> MLLHEFGLLESPKALEEAPWPPPEGAFVGFVLSRKEPMWADLLALAAARGGRVHRAPEPYKALRDLKEARGLLAKDLSVLALREGLGLPPGDDPMLLAYLLDPSNTTPEGVARRYGGEWTEEAGERAALSERLFANLWGRLEGEERLLWLYREVERPLSAVLAHMEATGVRLDVAYLRALSLEVAEEIARLEAEVFRLAGHPFNLNSRD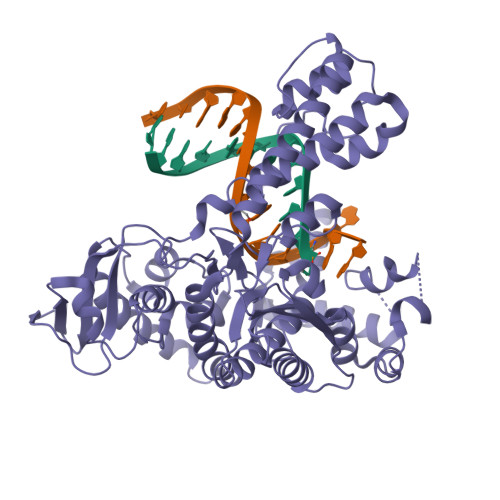QLERVLFDELGLPAIGKTEKTGKRSTSAAVLEALREAHPIVEKILQYRELTKLKSTYIDPLPDLIHPRTGRLHTRFNQTATATGRLSSSDPNLQNIPVRTPLGQRIRRAFIAEEGWLLVALDYSQIELRVLAHLSGDENLIRVFQEGRDIHTETASWMFGVPREAVDPLMRRAAKTINFGVLYGMSAHRLSQELAIPYEEAQAFIERYFQSFPKVRAWLEKTLEEGRRRGYVETLFGRRRYVPDLEARVKSVREAAERMAFNMPVQGTAADLMKLAMVKLFPRLEEMGARMLLQVHDELVLEAPKERAEAVARLAKEVMEGVYPLAVPLEVEVGIGEDWLSAKE> MAFVATQGATVVDQTTLMKKYLQFVAALTD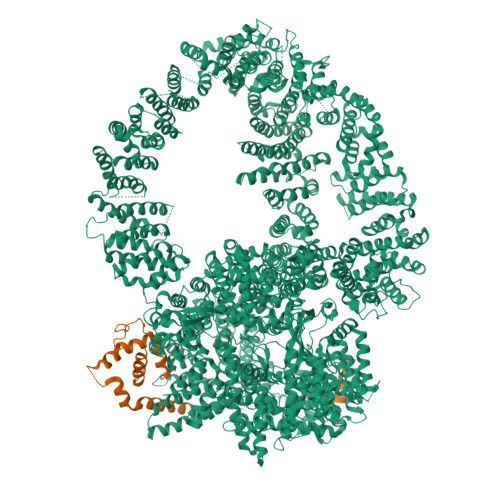VNTPDETKLKMMQEVSENFENVTSSPQYSTFLEHIIPRFLTFLQDGEVQFLQEKPAQQLRKLVLEIIHRIPTNEHLRPHTKNVLSVMFRFLETENEENVLICLRIIIELHKQFRPPITQEIHHFLDFVKQIYKELPKVVNRYFENPQVIPENTVPPPEMVGMITTIAVKVNPEREDSETRTHSIIPRGSLSLKVLAELPIIVVLMYQLYKLNIHNVVAEFVPLIMNTIAIQVSAQARQHKLYNKELYADFIAAQIKTLSFLAYIIRIYQELVTKYSQQMVKGMLQLLSNCPAETAHLRKELLIAAKHILTTELRNQFIPCMDKLFDESILIGSGYTARETLRPLAYSTLADLVHHVRQHLPLSDLSLAVQLFAKNIDDESLPSSIQTMSCKLLLNLVDCIRSKSEQESGNGRDVLMRMLEVFVLKFHTIARYQLSAIFKKCKPQSELGAVEAALPGVPTAPAAPGPAPSPAPVPAPPPPPPPPPPATPVTPAPVPPFEKQGEKDKEDKQTFQVTDCRSLVKTLVCGVKTITWGITSCKAPGEAQFIPNKQLQPKETQIYIKLVKYAMQALDIYQVQIAGNGQTYIRVANCQTVRMKEEKEVLEHFAGVFTMMNPLTFKEIFQTTVPYMVERISKNYALQIVANSFLANPTTSALFATILVEYLLDRLPEMGSNVELSNLYLKLFKLVFGSVSLFAAENEQMLKPHLHKIVNSSMELAQTAKEPYNYFLLLRALFRSIGGGSHDLLYQEFLPLLPNLLQGLNMLQSGLHKQHMKDLFVELCLTVPVRLSSLLPYLPMLMDPLVSALNGSQTLVSQGLRTLELCVDNLQPDFLYDHIQPVRAELMQALWRTLRNPADSISHVAYRVLGKFGGSNRKMLKESQKLHYVVTEVQGPSITVEFSDCKASLQLPMEKAIETALDCLKSANTEPYYRRQAWEVIKCFLVAMMSLEDNKHALYQLLAHPNFTEKTIPNVIISHRYKAQDTPARKTFEQALTGAFMSAVIKDLRPSALPFVASLIRHYTMVAVAQQCGPFLLPCYQVGSQPSTAMFHSEENGSKGMDPLVLIDAIAICMAYEEKELCKIGEVALAVIFDVASIILGSKERACQLPLFSYIVERLCACCYEQAWYAKLGGVVSIKFLMERLPLTWVLQNQQTFLKALLFVMMDLTGEVSNGAVAMAKTTLEQLLMRCATPLKDEERAEEIVAAQEKSFHHVTHDLVREVTSPNSTVRKQAMHSLQVLAQVTGKSVTVIMEPHKEVLQDMVPPKKHLLRHQPANAQIGLMEGNTFCTTLQPRLFTMDLNVVEHKVFYTELLNLCEAEDSALTKLPCYKSLPSLVPLRIAALNALAACNYLPQSREKIIAALFKALNSTNSELQEAGEACMRKFLEGATIEVDQIHTHMRPLLMMLGDYRSLTLNVVNRLTSVTRLFPNSFNDKFCDQMMQHLRKWMEVVVITHKGGQRSDGNESISECGRCPLSPFCQFEEMKICSAIINLFHLIPAAPQTLVKPLLEVVMKTERAMLIEAGSPFREPLIKFLTRHPSQTVELFMMEATLNDPQWSRMFMSFLKHKDARPLRDVLAANPNRFITLLLPGGAQTAVRPGSPSTSTMRLDLQFQAIKIISIIVKNDDSWLASQHSLVSQLRRVWVSENFQERHRKENMAATNWKEPKLLAYCLLNYCKRNYGDIELLFQLLRAFTGRFLCNMTFLKEYMEEEIPKNYSIAQKRALFFRFVDFNDPNFGDELKAKVLQHILNPAFLYSFEKGEGEQLLGPPNPEGDNPESITSVFITKVLDPEKQADMLDSLRIYLLQYATLLVEHAPHHIHDNNKNRNSKLRRLMTFAWPCLLSKACVDPACKYSGHLLLAHIIAKFAIHKKIVLQVFHSLLKAHAMEARAIVRQAMAILTPAVPARMEDGHQMLTHWTRKIIVEEGHTVPQLVHILHLIVQHFKVYYPVRHHLVQHMVSAMQRLGFTPSVTIEQRRLAVDLSEVVIKWELQRIKDQQPDSDMDPNSSGEGVNSVSSSIKRGLSVDSAQEVKRFRTATGAISAVFGRSQSLPGADSLLAKPIDKQHTDTVVNFLIRVACQVNDNTNTAGSPGEVLSRRCVNLLKTALRPDMWPKSELKLQWFDKLLMTVEQPNQVNYGNICTGLEVLSFLLTVLQSPAILSSFKPLQRGIAACMTCGNTKVLRAVHSLLSRLMSIFPTEPSTSSVASKYEELECLYAAVGKVIYEGLTNYEKATNANPSQLFGTLMILKSACSNNPSYIDRLISVFMRSLQKMVREHLNPQAASGSTEATSGTSELVMLSLELVKTRLAVMSMEMRKNFIQAILTSLIEKSPDAKILRAVVKIVEEWVKNNSPMAANQTPTLREKSILLVKMMTYIEKRFPEDLELNAQFLDLVNYVYRDETLSGSELTAKLEPAFLSGLRCAQPLIRAKFFEVFDNSMKRRVYERLLYVTCSQNWEAMGNHFWIKQCIELLLAVCEKSTPIGTSCQGAMLPSITNVINLADSHDRAAFAMVTHVKQEPRERENSESKEEDVEIDIELAPGDQTSTPKTKELSEKDIGNQLHMLTNRHDKFLDTLREVKTGALLSAFVQLCHISTTLAEKTWVQLFPRLWKILSDRQQHALAGEISPFLCSGSHQVQRDCQPSALNCFVEAMSQCVPPIPIRPCVLKYLGKTHNLWFRSTLMLEHQAFEKGLSLQIKPKQTTEFYEQESITPPQQEILDSLAELYSLLQEEDMWAGLWQKRCKYSETATAIAYEQHGFFEQAQESYEKAMDKAKKEHERSNASPAIFPEYQLWEDHWIRCSKELNQWEALTEYGQSKGHINPYLVLECAWRVSNWTAMKEALVQVEVSCPKEMAWKVNMYRGYLAICHPEEQQLSFIERLVEMASSLAIREWRRLPHVVSHVHTPLLQAAQQIIELQEAAQINAGLQPTNLGRNNSLHDMKTVVKTWRNRLPIVSDDLSHWSSIFMWRQHHYQGKPTWSGMHSSSIVTAYENSSQHDPSSNNAMLGVHASASAIIQYGKIARKQGLVNVALDILSRIHTIPTVPIVDCFQKIRQQVKCYLQLAGVMGKNECMQGLEVIESTNLKYFTKEMTAEFYALKGMFLAQINKSEEANKAFSAAVQMHDVLVKAWAMWGDYLENIFVKERQLHLGVSAITCYLHACRHQNESKSRKYLAKVLWLLSFDDDKNTLADAVDKYCIGVPPIQWLAWIPQLLTCLVGSEGKLLLNLISQVGRVYPQAVYFPIRTLYLTLKIEQRERYKSDPGPIRATAPMWRCSRIMHMQRELHPTLLSSLEGIVDQMVWFRENWHEEVLRQLQQGLAKCYSVAFEKSGAVSDAKITPHTLNFVKKLVSTFGVGLENVSNVSTMFSSAASESLARRAQATAQDPVFQKLKGQFTTDFDFSVPGSMKLHNLISKLKKWIKILEAKTKQLPKFFLIEEKCRFLSNFSAQTAEVEIPGEFLMPKPTHYYIKIARFMPRVEIVQKHNTAARRLYIRGHNGKIYPYLVMNDACLTESRREERVLQLLRLLNPCLEKRKETTKRHLFFTVPRVVAVSPQMRLVEDNPSSLSLVEIYKQRCAKKGIEHDNPISRYYDRLATVQARGTQASHQVLRDILKEVQSNMVPRSMLKEWALHTFPNATDYWTFRKMFTIQLALIGFAEFVLHLNRLNPEMLQIAQDTGKLNVAYFRFDINDATGDLDANRPVPFRLTPNISEFLTTIGVSGPLTASMIAVARCFAQPNFKVDGILKTVLRDEIIAWHKKTQEDTSSPLSAAGQPENMDSQQLVSLVQKAVTAIMTRLHNLAQFEGGESKVNTLVAAANSLDNLCRMDPAWHPWL;> MHHGTGPQNVQHQLQRSRACPGSEGEEQPAHPNPPPSPAAPFAPSASPSAPQSPSYQIQQLMNRSPATGQNVNITLQSVGPVVGGNQQITLAPLPLPSPTSPGFQFSAQPRRFEHGSPSYIQVTSPLSQQVQTQSPTQPSPGPGQALQNVRAGAPGPGLGLCSSSPTGGFVDASVLVRQISLSPSSGGHFVFQDGSGLTQIAQGAQVQLQHPGTPITVRERRPSQPHTQSGGTIHHLGPQSPAAAGGAGLQPLASPSHITTANLPPQISSIIQGQLVQQQQVLQGPPLPRPLGFERTPGVLLPGAGGAAGFGMTSPPPPTSPSRTAVPPGLSSLPLTSVGNTGMKKVPKKLEEIPPASPEMAQMRKQCLDYHYQEMQALKEVFKEYLIELFFLQHFQGNMMDFLAFKKKHYAPLQAYLRQNDLDIEEEEEEEEEEEEKSEVINDEVKVVTGKDGQTGTPVAIATQLPPKVSAAFSSQQQPFQQALAGSLVAGAGSTVETDLFKRQQAMPSTGMAEQSKRPRLEVGHQGVVFQHPGADAGVPLQQLMPTAQGGMPPTPQAAQLAGQRQSQQQYDPSTGPPVQNAASLHTPLPQLPGRLPPAGVPTAALSSALQFAQQPQVVEAQTQLQIPVKTQQPNVPIPAPPSSQLPIPPSQPAQLALHVPTPGKVQVQASQLSSLPQMVASTRLPVDPAPPCPRPLPTSSTSSLAPVSGSGPGPSPARSSPVNRPSSATNKALSPVTSRTPGVVASAPTKPQSPAQNATSSQDSSQDTLTEQITLENQVHQRIAELRKAGLWSQRRLPKLQEAPRPKSHWDYLLEEMQWMATDFAQERRWKVAAAKKLVRTVVRHHEEKQLREERGKKEEQSRLRRIAASTAREIECFWSNIEQVVEIKLRVELEEKRKKALNLQKVSRRGKELRPKGFDALQESSLDSGMSGRKRKASISLTDDEVDDEEETIEEEEANEGVVDHQTELSNLAKEAELPLLDLMKLYEGAFLPSSQWPRPKPDGEDTSGEEDADDCPGDRESRKDLVLIDSLFIMDQFKAAERMNIGKPNAKDIADVTAVAEAILPKGSARVTTSVKFNAPSLLYGALRDYQKIGLDWLAKLYRKNLNGILADEAGLGKTVQIIAFFAHLACNEGNWGPHLVVVRSCNILKWELELKRWCPGLKILSYIGSHRELKAKRQEWAEPNSFHVCITSYTQFFRGLTAFTRVRWKCLVIDEMQRVKGMTERHWEAVFTLQSQQRLLLIDSPLHNTFLELWTMVHFLVPGISRPYLSSPLRAPSEESQDYYHKVVIRLHRVTQPFILRRTKRDVEKQLTKKYEHVLKCRLSNRQKALYEDVILQPGTQEALKSGHFVNVLSILVRLQRICNHPGLVEPRHPGSSYVAGPLEYPSASLILKALERDFWKEADLSMFDLIGLENKITRHEAELLSKKKIPRKLMEEISTSAAPAARPAAAKLKASRLFQPVQYGQKPEGRTVAFPSTHPPRTAAPTTASAAPQGPLRGRPPIATFSANPEAKAAAAPFQTSQASASAPRHQPASASSTAASPAHPAKLRAQTTAQASTPGQPPPQPQAPSHAAGQSALPQRLVLPSQAQARLPSGEVVKIAQLASITGPQSRVAQPETPVTLQFQGSKFTLSHSQLRQLTAGQPLQLQGSVLQIVSAPGQPYLRAPGPVVMQTVSQAGAVHGALGSKPPAGGPSPAPLTPQVGVPGRVAVNALAVGEPGTASKPASPIGGPTQEEKTRLLKERLDQIYLVNERRCSQAPVYGRDLLRICALPSHGRVQWRGSLDGRRGKEAGPAHSYTSSSESPSELMLTLCRCGESLQDVIDRVAFVIPPVVAAPPSLRVPRPPPLYSHRMRILRQGLREHAAPYFQQLRQTTAPRLLQFPELRLVQFDSGKLEALAILLQKLKSEGRRVLILSQMILMLDILEMFLNFHYLTYVRIDENASSEQRQELMRSFNRDRRIFCAILSTHSRTTGINLVEADTVVFYDNDLNPVMDAKAQEWCDRIGRCKDIHIYRLVSGNSIEEKLLKNGTKDLIREVAAQGNDYSMAFLTQRTIQELFEVYSPMDDAGFPVKAEEFVVLSQEPSVTETIAPKIARPFIEALKSIEYLEEDAQKSAQEGVLGPHTDALSSDSENMPCDEEPSQLEELADFMEQLTPIEKYALNYLELFHTSIEQEKERNSEDAVMTAVRAWEFWNLKTLQEREARLRLEQEEAELLTYTREDAYSMEYVYEDVDGQTEVMPLWTPPTPPQDDSDIYLDSVMCLMYEATPIPEAKLPPVYVRKERKRHKTDPSAAGRKKKQRHGEAVVPPRSLFDRATPGLLKIRREGKEQKKNILLKQQVPFAKPLPTFAKPTAEPGQDNPEWLISEDWALLQAVKQLLELPLNLTIVSPAHTPNWDLVSDVVNSCSRIYRSSKQCRNRYENVIIPREEGKSKNNRPLRTSQIYAQDENATHTQLYTSHFDLMKMTAGKRSPPIKPLLGMNPFQKNPKHASVLAESGINYDKPLPPIQVASLRAERIAKEKKALADQQKAQQPAVAQPPPPQPQPPPPPQQPPPPLPQPQAAGSQPPAGPPAVQPQPQPQPQTQPQPVQAPAKAQPAITTGGSAAVLAGTIKTSVTGTSMPTGAVSGNVIVNTIAGVPAATFQSINKRLASPVAPGALTTPGGSAPAQVVHTQPPPRAVGSPATATPDLVSMATTQGVRAVTSVTASAVVTTNLTPVQTPARSLVPQVSQATGVQLPGKTITPAHFQLLRQQQQQQQQQQQQQQQQQQQQQQQQQQQQQTTTTSQVQVPQIQGQAQSPAQIKAVGKLTPEHLIKMQKQKLQMPPQPPPPQAQSAPPQPTAQVQVQTSQPPQQQSPQLTTVTAPRPGALLTGTTVANLQVARLTRVPTSQLQAQGQMQTQAPQPAQVALAKPPVVSVPAAVVSSPGVTTLPMNVAGISVAIGQPQKAAGQTVVAQPVHMQQLLKLKQQAVQQQKAIQPQAAQGPAAVQQKITAQQITTPGAQQKVAYAAQPALKTQFLTTPISQAQKLAGAQQVQTQIQVAKLPQVVQQQTPVASIQQVASASQQASPQTVALTQATAAGQQVQMIPAVTATAQVVQQKLIQQQVVTTASAPLQTPGAPNPAQVPASSDSPSQQPKLQMRVPAVRLKTPTKPPCQ N-[5'-O-PHOSPHONO-RIBOFURANOSYL]-2-[2-HYDROXY-2-[4-[GLUTAMIC ACID]-N-CARBONYLPHENYL]-3-[2-AMINO-4-HYDROXY-QUINAZOLIN-6-YL]-PROPANYLAMINO]-ACETAMIDE | C30 H37 N6 O15 P 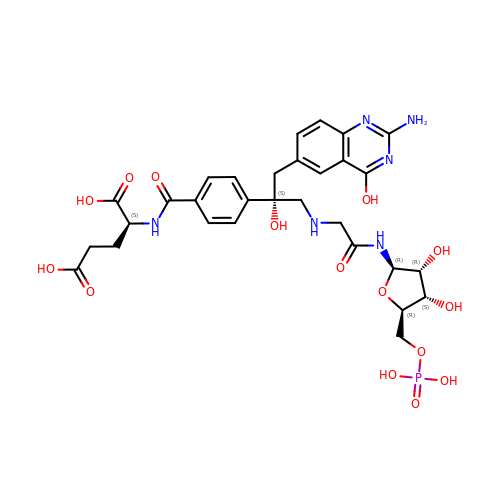| QZUCAWXKEZPFBV-PRICPSHJSA-N1~{H}-pyrazol-5-ylmethanol 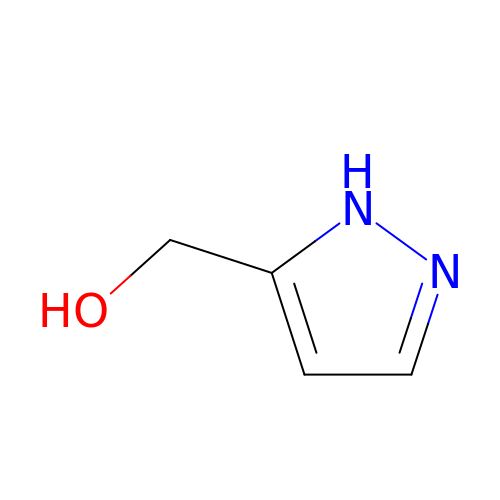| C4 H6 N2 O | UIEABCXJWANXFS-UHFFFAOYSA-N> MTSPQLEWTLQTLLEQLNEDELKSFKSLLWAFPLEDVLQKTPWSEVEEADGKKLAEILVNTSSENWIRNATVNILEEMNLTELCKMAKAEMMEDGQVQEIDNPELGDAEEDSELAKPGEKEGWRNSMEKQSLVWKNTFWQGDIDNFHDDVTLRNQRFIPFLNPRTPRKLTPYTVVLHGPAGVGKTTLAKKCMLDWTDCNLSPTLRYAFYLSCKELSRMGPCSFAELISKDWPELQDDIPSILAQAQRILFVVDGLDELKVPPGALIQDICGDWEKKKPVPVLLGSLLKRKMLPRAALLVTTRPRALRDLQLLAQQPIYVRVEGFLEEDRRAYFLRHFGDEDQAMRAFELMRSNAALFQLGSAPAVCWIVCTTLKLQMEKGEDPVPTCLTRTGLFLRFLCSRFPQGAQLRGALRTLSLLAAQGLWAQMSVFHREDLERLGVQESDLRLFLDGDILRQDRVSKGC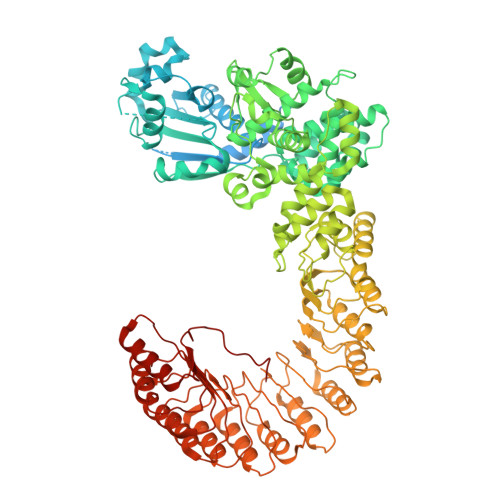YSFIHLSFQQFLTALFYALEKEEGEDRDGHAWDIGDVQKLLSGEERLKNPDLIQVGHFLFGLANEKRAKELEATFGCRMSPDIKQELLQCKAHLHANKPLSVTDLKEVLGCLYESQEEELAKVVVAPFKEISIHLTNTSEVMHCSFSLKHCQDLQKLSLQVAKGVFLENYMDFELDIEFERCTYLTIPNWARQDLRSLRLWTDFCSLFSSNSNLKFLEVKQSFLSDSSVRILCDHVTRSTCHLQKVEIKNVTPDTAYRDFCLAFIGKKTLTHLTLAGHIEWERTMMLMLCDLLRNHKCNLQYLRLGGHCATPEQWAEFFYVLKANQSLKHLRLSANVLLDEGAMLLYKTMTRPKHFLQMLSLENCRLTEASCKDLAAVLVVSKKLTHLCLAKNPIGDTGVKFLCEGLSYPDCKLQTLVLQQCSITKLGCRYLSEALQEACSLTNLDLSINQIARGLWILCQALENPNCNLKHLRLWSCSLMPFYCQHLGSALLSNQKLETLDLGQNHLWKSGIIKLFGVLRQRTGSLKILRLKTYETNLEIKKLLEEVKEKNPKLTIDCNASGATAPPCCDFFC> SNAMSNELRLEDNYVPTSDTLVVFKQLMKLPVTVLYDLTLSWFAKFGGSFDGDIYLLTETLDLLIEKGVRRNVIVNRILYVYWPDGLNVFQLAEIDCHLMISKPEKFKWLPSKALRGDGKPYVVKLQPAKFIENLQTDLAKIYHCHVYMFKHPSLPVLITRIQLFDSNNLFLSTPNIGSINKESLYNKLDKFQGKPLISRRPYYVAFPLNSPIIFHSVDKDIYARLVLQSISRTISERETIIFKPVQKIPVKSIHNIMTLLGPSRFAESMGPWECYASANFERSPLHDYKKHQGLTGKKVMVREFDDSFLNDDENFYGKEEPEIRRLRLEKNMIKFKGSANGVMDQKYNDL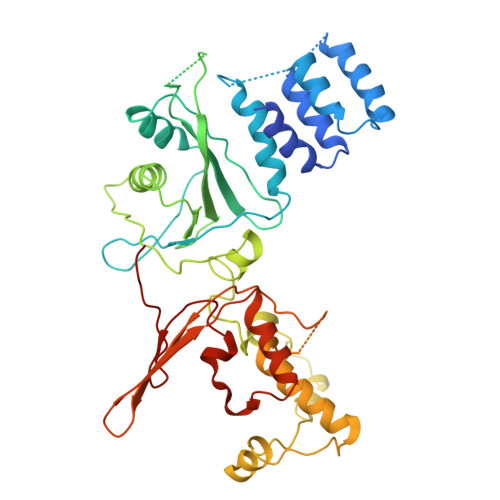KEFNEHVHNIRNGKKNEDSGEPVYISRYSSLVPIEKVGFTLKNEINSRIITIKLKFNGNDIFGGLHELCDKNLINIDKVPGWLAGENGSFSGTIMNGDFQREQVAKGGLL> GLDRNRQDIGYVLGRLFAVLEKIQAEANPGLNATIADRYFGSASSTPIAVFGTLMRLLPHHLNKLEFEGRAVQLQWEIRQILEHCQRFPNHLNLEQQGLFAIGYYHETQFLFTKDALKN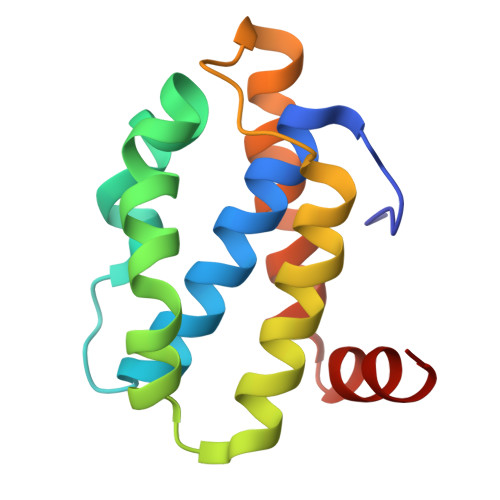LFNEA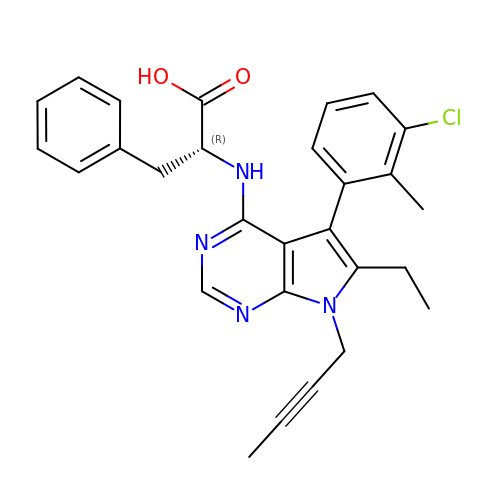(2~{R})-2-[[7-but-2-ynyl-5-(3-chloranyl-2-methyl-phenyl)-6-ethyl-pyrrolo[2,3-d]pyrimidin-4-yl]amino]-3-phenyl-propanoic acid | C28 H27 Cl N4 O2 | PMJJSYCWIFTUKH-JOCHJYFZSA-N>YIIPDEIPYKAVVNIENIVATVTLDQTLDLYAMERSVPNVEYDPDQFPGLIF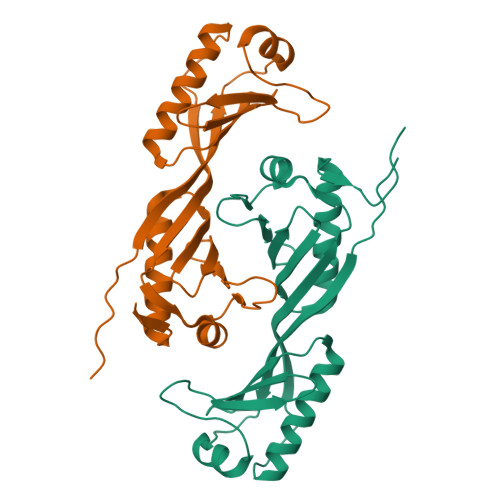RLESPKITSLIFKSGKMVVTGAKSTDELIKAVKRIIKTLKKYGMQLTGKPKIQIQNIVASANLHVIVNLDKAAFLLENNMYEPEQFPGLIYRMDEPRVVLLIFSSGKMVITGAKREDEVHKAVKKIFDKLVELDCVKPVEEEELEF[2x]>MSYQPQTEAATSRFL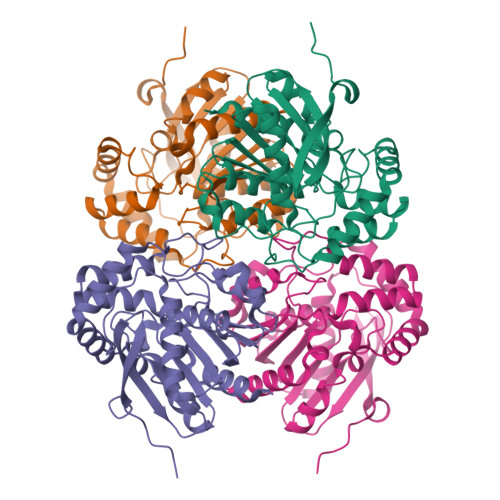NVEEAGKTLRIHFNDCGQGDETVVLLHGSGPGATGWANFSRNIDPLVEAGYRVILLDCPGWGKSDSVVNSGSRSDLNARILKSVVDQLDIAKIHLLGNSMGGHSSVAFTLKWPERVGKLVLMGGGTGGMSLFTPMPTEGIKRLNQLYRQPTIENLKLMMDIFVFDTSDLTDALFEARLNNMLSRRDHLENFVKSLEANPKQFPDFGPRLAEIKAQTLIVWGRNDRFVPMDAGLRLLSGIAGSELHIFRDCGHWAQWEHADAFNQLVLNFLARP[4x]>[2x]MVLYFIGLGLYDERDITVKGLEIAKKCDYVFA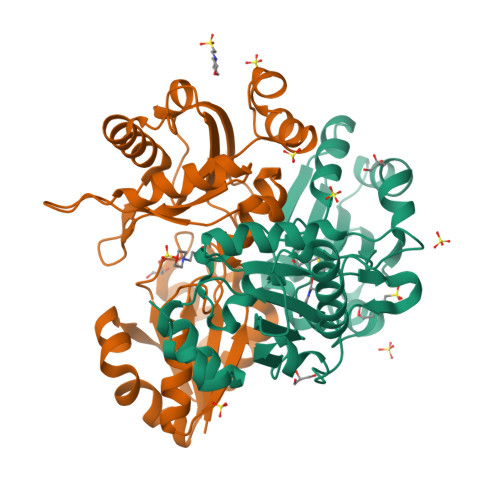EFYTSLMAGTTLGRIQRLIGKEIRVLSREDVELNFENIVLPLAKENDVAFLTPGDPLVATTHAELRIRAKRAGVESYVIHAPSIYSAVGITGLHIYKFGKSATVAYPEGNWFPTSYYDVIKENAERGLHTLLFLDIKAEKRMYMTANEAMELLLKVEDMKKGGVFTDDTLVVVLARAGSLNPTIRAGYVKDLIREDFGDPPHILIVPGKLHIVEAEYLVEIAGAPREILRVNV> 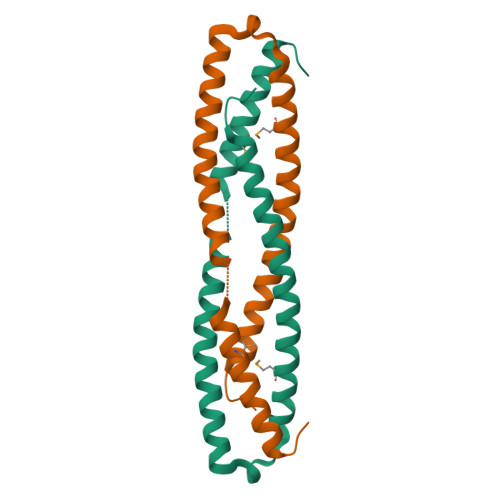AAISNLIPKLGELLTEEFKLHKGVKKNIEDLGKELESMNAALIKIGEVPREQLDSQDKLWADEVRELSYVIEDVVDKFLVQVDGIKSDDNNNKFKGLMKRTTELLKKVKHKHGIA4-cyclopropylbenzoic acid | C10 H10 O2 | 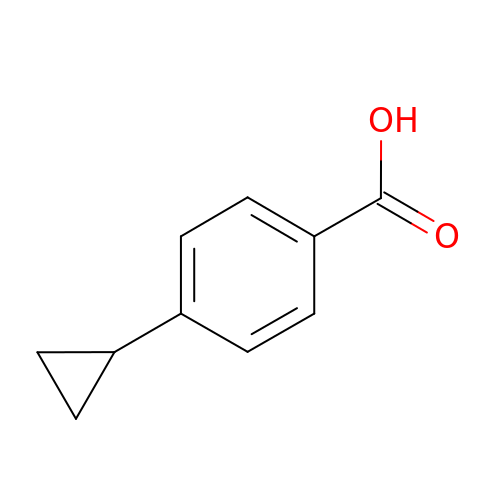GJCRWEAWEDESNZ-UHFFFAOYSA-N> GSVDMPLTEHLRELRYRLIISIIAFLIGSGIAFYFAKYVFEILAAPILKSYPEVELITLSPTEPLFILIKISLAVGFIIASPVILYQFWRFIEPALYSHEKRAFIPLLLGSILLFMLGALFAYFIVLPLALKFLLGLGFTQLLATPYLSVDMYISFVLKLVVAFGIAFEMPIVLYVLQKAGVITPEQLASF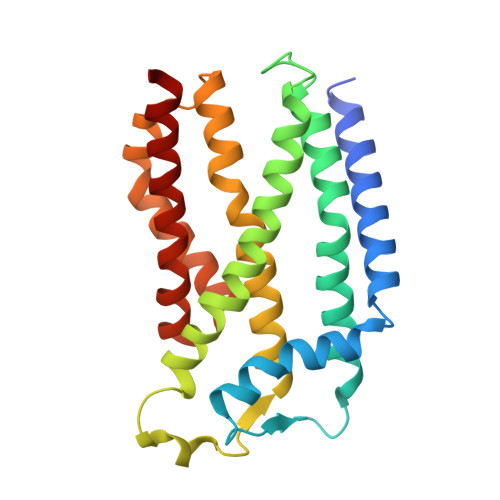RKYFIVIAFVIGAIIAPDVSTQVLMAIPLLLLYEISIFLGKLATR>MKVWLVGAYGIVSTTAMVGARAIERGIAPKIGLVSELPHFEGIEKYAPFSFEFGGHEIRLLSNAYEAAKEHWELNRHFDREILEAVKSDLEGIVARKGTALNCGSGIKELGDI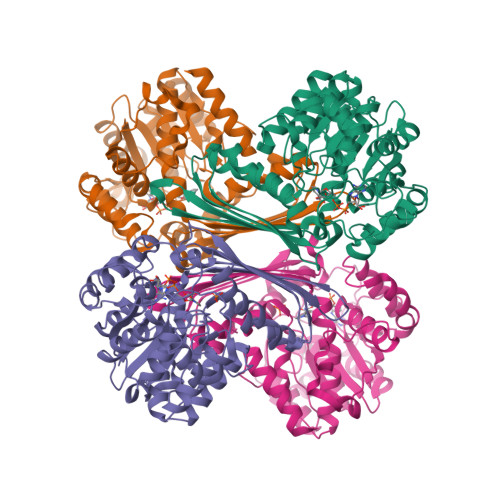KTLEGEGLSLAEMVSRIEEDIKSFADDETVVINVASTEPLPNYSEEYHGSLEGFERMIDEDRKEYASASMLYAYAALKLGLPYANFTPSPGSAIPALKELAEKKGVPHAGNDGKTGETLVKTTLAPMFAYRNMEVVGWMSYNILGDYDGKVLSARDNKESKVLSKDKVLEKMLGYSPYSITEIQYFPSLVDNKTAFDFVHFKGFLGKLMKFYFIWDAIDAIVAAPLILDIARFLLFAKKKGVKGVVKEMAFFFKSPMDTNVINTHEQFVVLKEWYSNLK[4x]(4-chlorophenyl)methyl pyridine-3-carboxylate 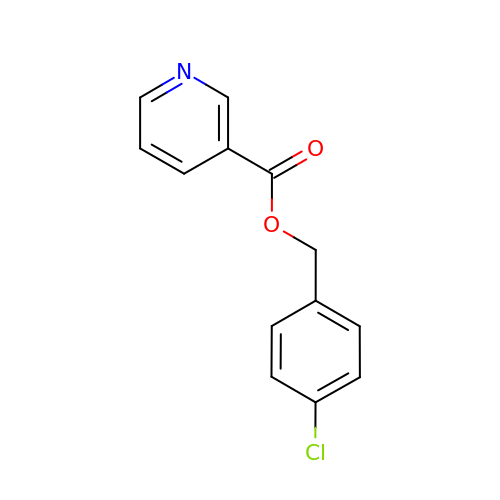| C13 H10 Cl N O2 | FLUZHFKASOGKOP-UHFFFAOYSA-N> KI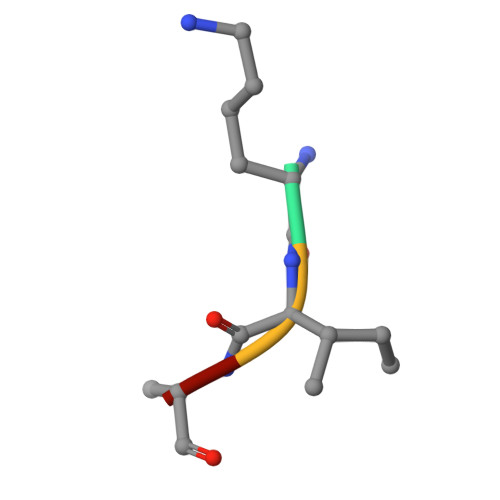AA>[4x]LHRNSLIVLADVALFLALYHFLPFEHNVVLGISMLAFIAVLWLTEALHVTVTAILVPVMAVFFGIFETQAALNNFANSIIFLFLGGFALAAAMHHQGLDKVIADKVLAMAQGKMSVAVFMLFGVTALLSMWISNTATAAMMLPLVLGVLSKVDADKQRSTYVFVLLGVAYSASIGGIATLVGSPPNAIAAAEVGLSFTDWMKFGLPTAMMMLPMAIAILYFLLKPTLNGMFELDRAPVNWDKGKVVTLGIFGLTVFLWIFSSPINAALGGFKSFDTLVALGAILMLSFARVVHWKEIQKTADWGVLLLFGGGLCLSNVLKQTGTSVFLANALSDMVSHMGIFVVILVVATFVVFLTEFASNTASAALLIPVFATVAEAFGMSPVLLSVLIAVAASCAFMLPVATPPNAIVFASGHIKQSEMMRVGLYLNIACIGLLTAIAMLFWQ

Membrane transporters belonging to the ubiquitous divalent anion/Na+ symporter (DASS) family move Krebs cycle intermediates or sulphate across the cell membrane typically by utilizing the preexisting Na+ gradient. However, like other well-characterized bacterial DASS proteins, VcINDY is known to transport succinate and other C4-dicarboxylates, rather than citrate (C6-tricarboxylate)1319. Our structure reveals a homodimeric arrangement, with each VcINDY protomer comprising eleven membrane-spanning helices (TM1–TM11), two re-entrant helix-turn-helix hairpins (HPin and HPout) and two interfacial helices (H4c and H9c). Viewed in parallel to the membrane, the VcINDY dimer is shaped like an inverted bowl with its concave mouth facing the cytoplasm, allowing the aqueous solution to reach the midpoint of the membrane.

To uncover how VcINDY distinguishes between C4-dicarboxylate and C6-tricarboxylate, we determined the structure of a citrate-bound VcINDY. Citrate inhibits the VcINDY-mediated succinate transport, likely as a competitive inhibitor. In the citrate-bound VcINDY, the side-chain amide of N151 and the side-chain hydroxyl of T152 donate H-bonds to a terminal carboxylate (pro-R) of the bound citrate, whereas the side-chain hydroxyl of S377 and the side-chain amide of N378 form H-bonds with the central carboxylate of citrate. Moreover, the side chains of P201, V322 and T379 make van der Waals interactions with the bound citrate. One terminal carboxylate (pro-S) and the hydroxyl of citrate, however, make no interaction with VcINDY and project towards the solvent. More importantly, our co-structure indicated that the citrate- and succinate-binding sites overlap substantially in VcINDY, and that citrate inhibits the transport of succinate by preoccupying the substrate-binding site, that is, as a competitive inhibitor. In our VcINDY structures, the two carboxylates of succinate occupy virtually the same position as the central and pro-R carboxylates of citrate. In the citrate-bound structure, the pro-S carboxylate, which probably carries a full negative charge (crystallization pH∼7), makes no interaction with VcINDY. Rather, P201, V322 and T379 pack against the bound citrate and steer the pro-S carboxylate away from the transporter. Therefore, the negative charges in citrate may not be fully ‘neutralized' by its interactions with VcINDY in the membrane bilayer. This finding may explain why citrate is less effective in inhibiting VcINDY-mediated succinate transport than C4-dicarboxylates and why citrate preferably binds to the inward-facing VcINDY.>[2x]AISSALPTIPYHKLADLRYLSRGASGTVSSARHADWRVQVAVKHLHIHTPLLDSERKDVLREAEILHKARFSYILPILGICNEPEFLGIVTEYMPNGSLNELLHRKTEYPDVAWPLRFRILHEIALGVNYLHNMTPPLLHHDLKTQNILLDNEFHVKIADFGLCKWRMMSLSQSRSSKSAPEGGTIIYMPPENYEPGQKSRASIKHDIYSYAVITWEVLSRKQPFEDVTN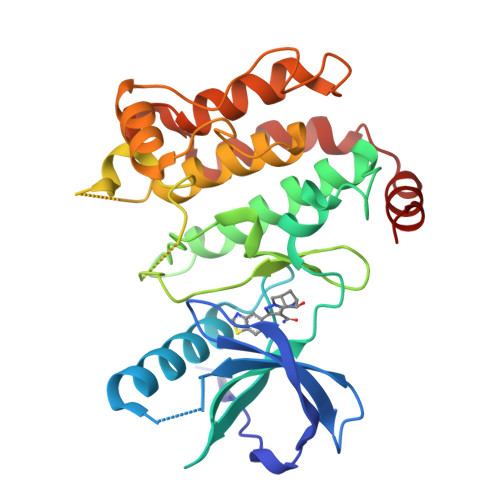PLQIMYSVSQGHRPVINEESLPYDIPHRARMISLIESGWAQNPDERPSFLKCLIELEPVLRTFEEITFLEAVIQLK>[30x]MAQSSNSTHEPLEVLKEETVNRHRAIVSVMEALEAVDWYDQRVDASTDPELTAILAHNRDEEKEHAAMTLEWLRRNDAKWAEHLRTYLFTEGPITAANSSSVDKLAAALEHHHHHH

Our study reports on a new class of ferritin-like proteins (EncFtn), which are associated with bacterial encapsulin nanocompartments (Enc). By studying the EncFtn from R. rubrum we demonstrate that iron binding results in assembly of EncFtn decamers, which display a unique annular architecture. Biochemical assays show that EncFtn is active as a ferroxidase enzyme. While EncFtn does not store iron itself, its association with the encapsulin nanocage suggests that mineralization occurs within the cavity of the encapsulin shell (McHugh et al., 2014).

Through site-directed mutagenesis we show that the conserved glutamic acid and histidine residues in the FOC influence protein assembly and activity. Analysis of each of the single mutations (E32A, E62A and H65A) made in the FOC highlights the importance of the iron-coordinating residues in the catalytic activity of EncFtn.4-(3-methylphenyl)-5-(1,5-naphthyridin-2-yl)-1,3-thiazol-2-amine | 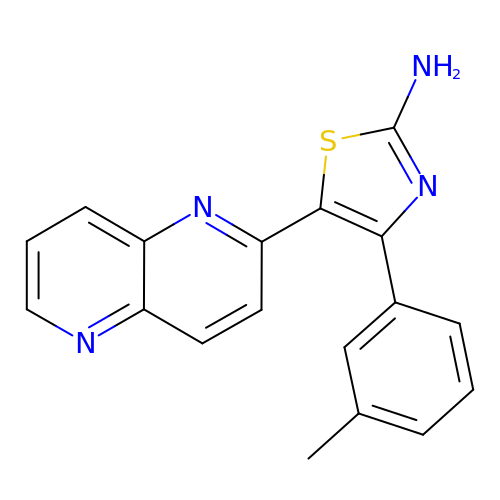C18 H14 N4 S | DKLCXLVLUXDLJI-UHFFFAOYSA-N> MELSSLTAVSPVDGRYGDKVSALRGIFSEYGLLKFRVQVEVRWLQKLAAHAAIKEVPAFAADAIGYLDAIVASFSEEDAARIKTIERTTNHDVKAVEYFLKEKVAEIPELHAVSEFIHFACTSEDINNLSHALMLKTARDEVILPYWRQLIDGLKDLAVQYRDIPLLSRTHGQPATPSTIGKEMANV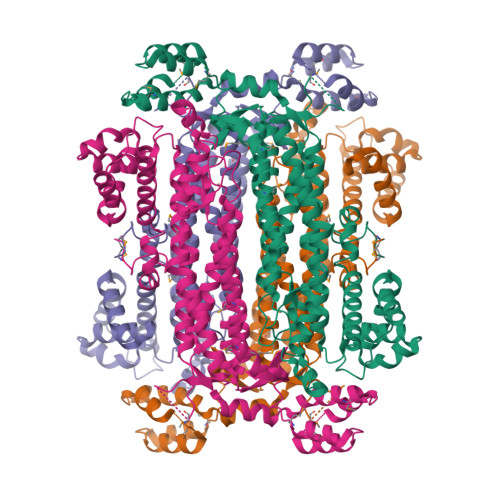AYRMERQYRQLNQVEILGKINGAVGNYNAHIAAYPEVDWHQFSEEFVTSLGIQWNPYTTQIEPHDYIAELFDCVARFNTILIDFDRDVWGYIALNHFKQKTIAGEIGSSTMPHKVNPIDFENSEGNLGLSNAVLQHLASKLPVSRWQRDLTDSTVLRNLGVGIGYALIAYQSTLKGVSKLEVNRDHLLDELDHNWEVLAEPIQTVMRRYGIEKPYEKLKELTRGKRVDAEGMKQFIDGLALPEEEKARLKAMTPANYIGRAITMVDELKHHHHHH>[2x]GSMTISNMEADCNRLLKQREELTKRREKLSKRREKIVKENGEGDKNVANINEEMESLTANIDYINDSISDCQANIMQMEEAK

Coiled-coils are important protein–protein interaction motifs present in ∼3% of all eukaryotic proteins. They consist of two or more amphipathic α-helices that wrap around each other’s hydrophobic seams resulting in parallel or antiparallel filamentous supercoils. Here, we present a case study for the phase determination of coiled-coil structures using a combination of native or engineered cysteine crosslinking together with native SAD phasing. In conclusion, our case study shows that cysteine crosslinking and phasing via sulfur-SAD is a particular useful strategy to solve coiled-coil structures by X-ray crystallography.

As a second case, we used the regulatory coiled-coil domain of the human kinesin-4 motor protein KIF21A. A recent study showed that the minimal KIF21A regulatory region folds into an intramolecular antiparallel coiled-coil monomer in solution, but crystallized into a dimeric domain-swapped antiparallel coiled-coil. Here, we aimed to stabilize and crystallize the native, monomeric coiled-coil form of the KIF21A regulatory region by rationally introducing cysteine residues (the construct is hereafter referred to as Kif21a_M947C). In the second case, Kif21a_M947C, we recombinantly introduced a cysteine residue to stabilize and crystallize the native, monomeric coiled-coil from the KIF21A regulatory region. A schematic representation of the KIF21A intramolecular antiparallel coiled-coil (amino acids 938–1017) is provided in Figure 2A, illustrating that a native cysteine, Cys1006, is present in a heptad repeat d core position. We therefore introduced the cysteine mutation in the juxtaposed heptad acore position of the coiled-coil to allow for disulfide bridge formation. The stability of Kif21a_M947C was assessed by thermal unfolding profiles monitored by CD at 222 nm, which yielded a Tm value of 37°C under reducing and 69°C under oxidizing conditions. As expected Kif21a_M947C was found to be monomeric under both reducing and oxidizing conditions (measured molecular mass: 11.3 kDa; calculated molecular mass: 9.5 kDa). The Kif21a_M947C coiled-coil fragment was crystallized under oxidizing buffer conditions. The final structure is composed of two intramolecular antiparallel coiled-coils per asymmetric unit with a disulfide bond between Cys947 and Cys1006. The results revealed the classical knobs into holes packing mode with the pairing of heptad a and d positions forming d/a mixed layers typical of antiparallel coiled-coils.BETA-ALANINE | C3 H7 N O2 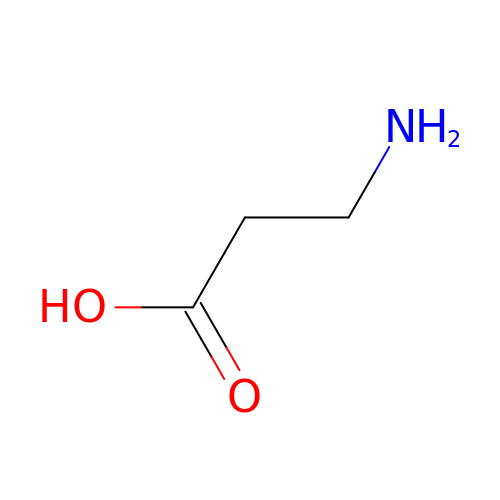| UCMIRNVEIXFBKS-UHFFFAOYSA-N>EKFKVITTFTVIADMAKNVAGDAAEVSSITKPGAEIHEYQPTPGDIKRAQGAQLILANGLNLERWFARFYQHLSGVPEVVVSTGVKPMGITEGPYNGK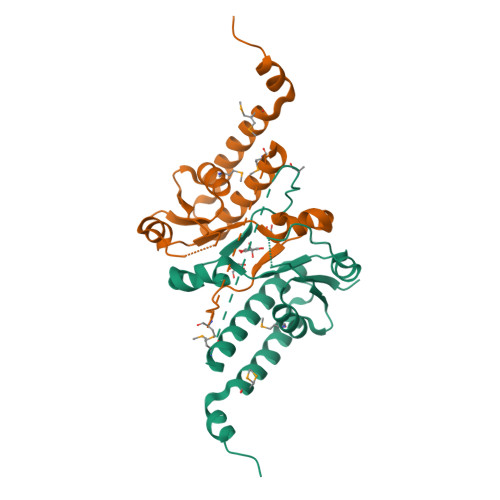PNPHAWMSAENALIYVDNIRDALVKYDPDNAQIYKQNAERYKAKIRQMADPLRAELEKIPAD[2x]>MSFLTLKDVDLKDKKVLVRVDFNVPVKDGKVTSKVRIEAAIPTIQYILDQGGAVILMSHLGRPTEGEYDSQFSLEPVAKALSEIINKPVKFAKDWLDGVDVKAGEIVMCENVRFNSGEKKSTDDLSKKIASLGDVFVMDAFATAHRAQASTYGVAKYIPVACAGILLTNEIQALEKALKSPKKPMAAIVGGSKVSTKLSVLNNLLDKVEILIVGGGIANTFIKAEGFDVGNSLYEQDLVAEATEILAKAKALGVNIPVPVDVRVAKEFSENAQAIIKKVSDVVADEMILDIGPESQKIIAELLKSANTILWNGPVGVFEFDNFAEGTKALSL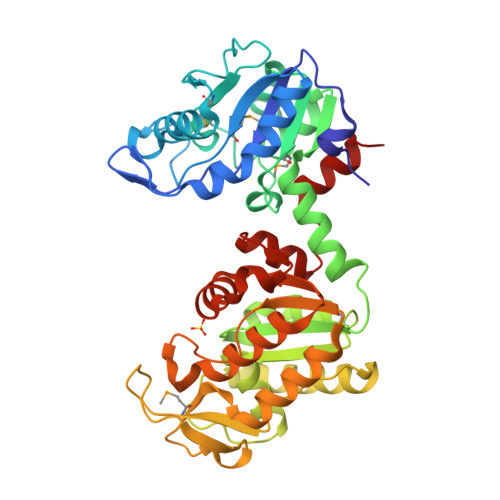AIAQSHAFSVAGGGDTIAAIEKFGIKDQVSYISTAGGAFLEFLEGKKLPAIEILKEKAIR[2x]>[2x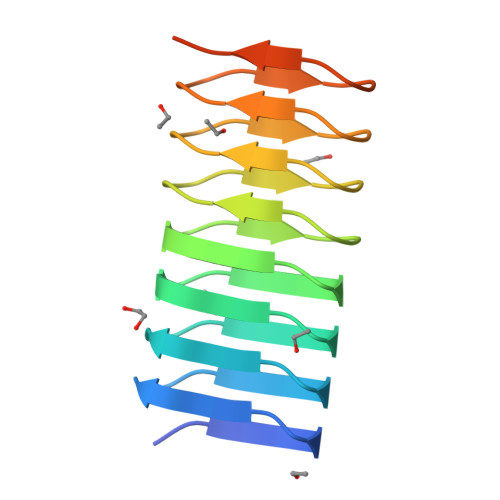]MDEQPNTISGSNNTVRSGSKNVLAGNDNTVISGDNNSVSGSNNTVVSGNDNTVTGSNHVVSGTNHIVTDNNNNVSGNDNNVSGSFHTVSGGHNTVSGSNNTVSGSNHVVSGSNKVVTDAAKLAAALEHHHHHH>[2x]MGLNDNKAGMEGLDKEKINKIIMEATKGSRFYGNELKKEKQVNQRIENMMQQKAQITSQQLRKAQLQVDRFAMELEQSRNLSNTIVHIDMDAFYAAVEMRDNPELKDKPIAVGSMSMLSTSNYHARRFGVRAAMPGFIAKRLCPQLIIVPPNFDKYRAVSKEVKEILADYDPNFMAMSLDEAYLNITKHLEERQNWPEDKRRYFIKMGSSVENDNPGKEVNKLSEHERSISPLLFEESPSDVQPPGDPFQVNFEEQNNPQILQNSVVFGTSAQEVVKEIRFRIEQKTTLTASAGIAPNTMLAKVCSDKNKPNGQYQILPNRQAVMDFIKDLPIRKVSGIGKVTEKMLKALGIITCTELYQQRALLSLL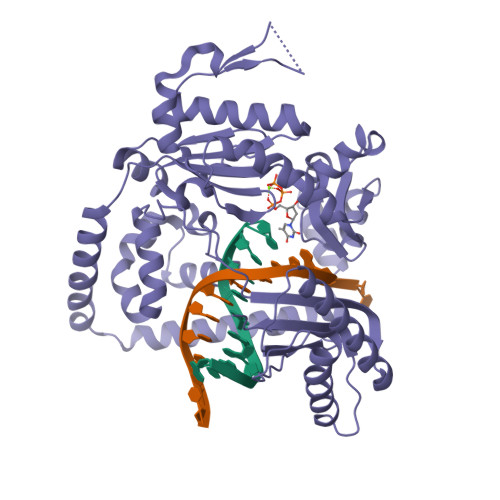FSETSWHYFLHISLGLGSTHLTRDGERKSMSVERTFSEINKAEEQYSLCQELCSELAQDLQKERLKGRTVTIKLKNVNFEVKTRASTVSSVVSTAEEIFAIAKELLKTEIDADFPHPLRLRLMGVRISSFPNEEDRKHQQ>GASSNKLFPPQIKVAATYMRGGTSKGVFFRLQDLPEAAQVPGPARDALLLRVIGSPDPYAKQIDGMGGATSSTSETVILSHSSKANHDVDYLFGQVSIDKPFVDWSGNCGNLTAAVGAFAISNGLIDAARIPRNGVCTVRIWQANIGKTIIAHVPITDGAVQETGDFELDGVTFPAAEVQIEFMNPAADDDGEGGCMFPTGNLVDVLEVPGIGRFNATMINAGIPTIFINAEDLGYTGTELQDDINSDNAALAKFETIRAHGA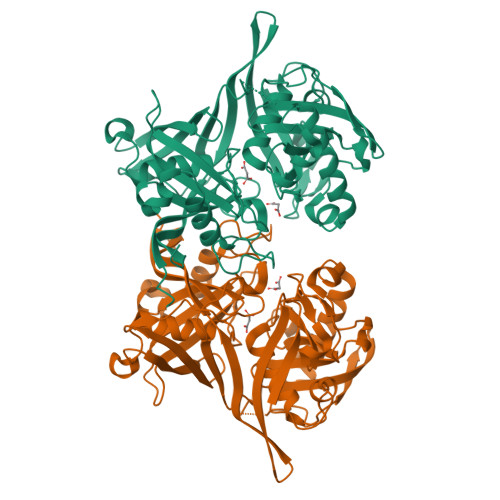LRMGLIKHIDEAASRQHTPKIAFVAPPKSYASSSGKTVAAEDVDLLVRALSMGKLHHAMMGTAAVAIGTAAAIPGTLVNLAAGGGEKEAVRFGHPSGTLRVGAQAVQENGEWTVIKAIMSRSARVLMEGFVRVPKP[2x]>SMSGMKSSKSKDVLSAAEVMQWSQSLEKLLANQTGQNVFGSFLKSEFSEENIEFWLACEDYKKTESDLLPCKAEEIYKAFVHSDAAKQIN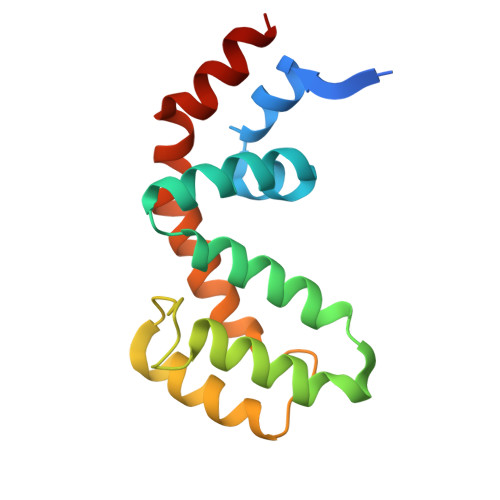IDFRTRESTAKKIKAPTPTCFDEAQKVIYTLMEKDSYPRFLKSDIYLNLLNDLQA[2x]> SNAMAASEPYTWKNVVIGGGGYVTGIIYHPNQSGLVYARTDIGGAYRWDSATSQWIPITDMLNRNNSDYMGILSIAIDPNDVNRVYMLCGKYTQSWAGTGAVLASTDKGATWTIYPLSVKIGGNEDGRGLGERLQVDPNLGSILFMGTTRDGLWKSTDRGATWVRVTSFTPTNINFVIFDKSSSSLGQATKRIFVGVNDTSGQSLWRSDDGGNTWKVVAGQPTGVMAMKAEIASGYLYVTFANSPGPNNATAGSVWRYTISNGEWKDISPAKGSYGYCGISVDPRNPNHILVATLDLWWPRDQIWRTTDGGSTWTPLLWNPSNNAVIAKFDTSSAPWAAIRNPHWITDIKIDPFNSNKAMFVTGYGIWACDNLSASPTTWYFRNKGLEEMVPIEIVSP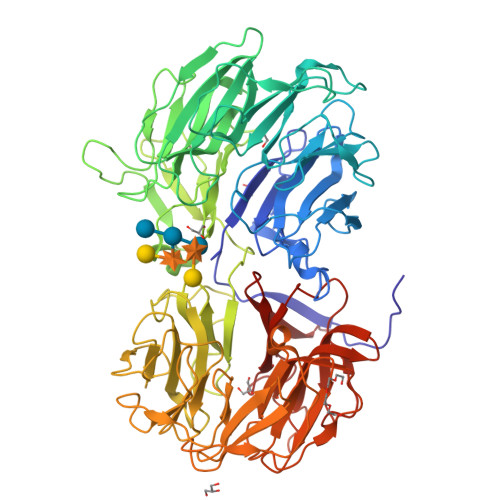PSGALLLSAMGDQGVFRHDSLDASPSMGVALDVGTAGSIDYAESIPSKIVATYYSAPYGAYSTDGGKTWTKFASYPAGTTGGGTRAIAISADGNRIVWAPNGAPMSYSTNNGSSWTTCGGGVPSGLSVEADKVNSNKFYAYDPVNGKLWVSTNGGVSFTQMSTSYPTLPSWQAYNGSVNAVFGREGDIWITCGAGGLYHSTNSGASATKVNSVQEAYSIGFGKAKTSGGYPAIYLHGIVNGVLGIFRSDDGGSTWTRINDDNHQFGWIHMIRGDQRTYGLCYVSAEGRGVIYGLPTPT>[2x]UUGGGCCAGCAGCAGGUCC

More than 15 neurological diseases are known to be caused by the expansion of these trinucleotide repeats, and the majority of a group of diseases are caused by the expansion of CAG repeats. Mutant transcript-mediated toxicity is due to the sequestration of regulatory proteins and factors by CAG repeat motifs e.g., muscleblind-like1 (MBNL1), a splicing regulator protein, nucleolin, a nucleolar protein and many other transcription factors. Over the past decade, the structural characteristics of RNAs containing CAG repeat motifs were explored by biochemical methods. These studies have shown that the long CAG repeat tracts form stable hairpins in which the C-G and G-C bases form closing pairs, and the A-A pairs interact within hairpins by forming 1x1 nucleotide internal loops. Here, we report the crystal structure of an RNA model containing three consecutive 5´-CAG/3´-GAC motif, which is complemented by an NMR-based solution structure and restrained Molecular Dynamics (rMD) simulation studies.

The duplex crystallised in the double-stranded helical structure and the structure was refined to resolution of 2.3 Å. The RNA duplex was constructed to contain 5´ UU dangling ends and a duplex region flanking the three CAG motifs. The central AA internal loop and one of the terminal 1x1 nucleotide AA internal loops have both adenines in an anti conformation. Despite being in the anti conformation, one of the A's in the central AA internal loop was slightly tilted and did not have well-defined electron density. In addition, the third AA internal loop had one of the A’s in the syn conformation with the other in the anti conformation. Two of the three 1x1 nucleotide AA internal loops have a zero hydrogen bond conformation, while the remaining loop has a single hydrogen bond conformation. In one hydrogen bond geometry, the hydrogen bond is between the hydrogen atom of the exocyclic amine (N6) of A14 and the N1 atom of A8. However, the X-ray crystal results here show that the syn-anti conformational change in the adenines was independent of Na+ ions. The C1´-C1´ distances between the CG closing pairs averaged 10.5 Å, whereas the distance between the AA pairs is greater than the standard distance of 10.5 Å. This observation explains the global widening of the major grooves of RNA as purine-purine pairs increases C1´-C1´ distances to 12.7 Å. Further, our crystal structure shows A'- form RNA due to the effect of base inclination and widening of major groove in CAG motif.>[2x]MRGSHHHHHHGSENLYFQDFTSLETTTFEEVVIALGSNVGNRMNNFKEALRLMKDYGISVTRHSCLYETEPVHVTDQPRFLNAAIRGVTKLKPHELLNVLKKIEKEMGREENGLRYGPRPLDLDILFYGK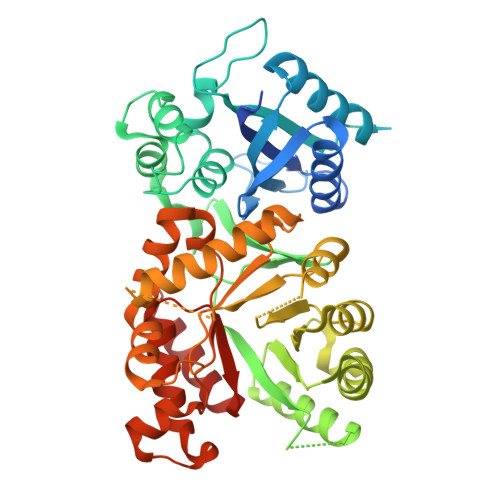HKIISDKLIIPHERIWERPFVLAPLVDLLGTEDIDNDKIVAYWHSLSMHSGGIFQAWERLGGESLLGKDGIIQRVIPIGDHLWDFSKKTYVMGILNLTPDSFSDGGKFQSVDTAVSRVRSMISEGVDIIDIGAQSTRPMASRISSQEEIDRLIPVLKVVRGMAEMKGKLISVDTFNSEVALEAIRNGADILNDVSGGSLDENMHKVVADSDVPYMIMHMRGDPCTMQNKENLEYNEICKDVATELYERVREAELSGIPAWRIMIDPGIGFSKGIDHNLDIVMELPKIREEMAKKSIGLSHAPILIGPSRKRFLGDICGRPEASERDAATVACVTAGILKGANIIRVHNVRDNVDAARLCDAMMTKRFKNVD>[2x]GPAMLPISMSDEGDSFLVKDSLGENKIPKNPSKVVILDLGILDTFDALKLNDKVVGVPAKNLPKYLQQFKNKP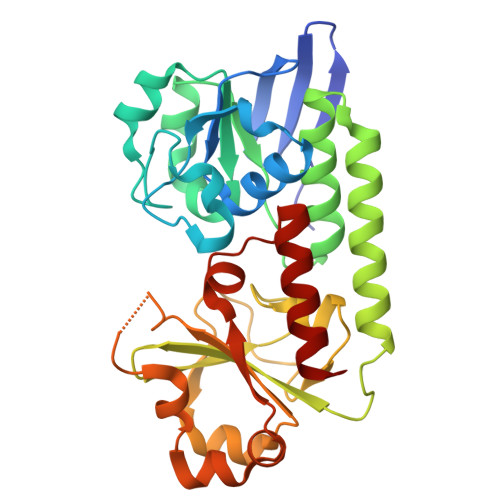SVGGVQQVDFEAINALKPDLIIISGRQSKFYDKLKEIAPTLFVGLDNANFLSSFENNVLSVAKLYGLEKEALEKISDIKNEIEKAKSIVDEDKKALIILTNSNKISAFGPQSRFGIIHDVLGINAVDENIKVGTAGKSINSEFILEKNPDYIFVVDRNVILGNKERAQGILDNALVAKTKAAQNKKIIYLDPEYWFLASGNGLESLKTMILEIKNAVK;> GPAMLPISMSDEGDSFLVKDSIGENKIPKNPSKVVILDLGILDTFDALKLNDKVVGVPAKNLPKYLQQFKNKPSVGGVQQVDFEAINALKPDLIIISGRQSKFYDKLKEIAPTLFVGLDNANFLSSFENNVLSVAKLYGLEKEALEKISDIKNEIEKAKSIVDEDKKALIILTNSNKISAFGPQSRFGIIHDVLGINAVDENIKVGTAGKSINSEFILEKNPDYIFVVDRNVILGNKERAQGILDNALVAKTKAAQNKKIIYLDPEYWFLASGNGLESLKTMILEIKNAVK> SVMTLLQLPDPTTDLPR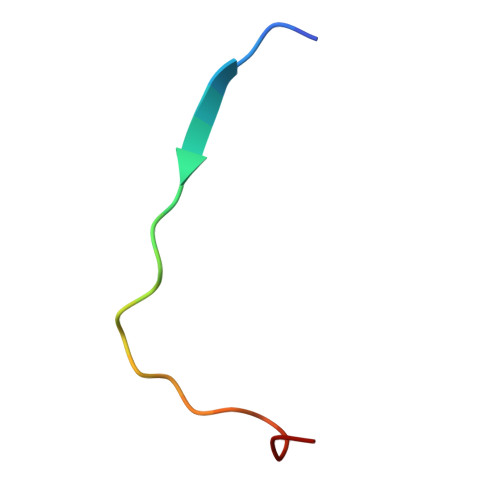EKPLP>MGSSHHHHHSSGENLYFQGHMSIPFTRWPEEFARRYREKGYWQDLPLTDILTRHAASDSIAVIDGERQLSYRELNQAADNLACSLRRQGIKPGETALVQLGNVAELYITFFALLKLGVAPVLALFSHQRSELNAYASQIEPALLIADRQHALFSGDDFLNTFVTEHSSIRVVQLLNDSGEHNLQDAINHPAEDFTATPSPADEVAYFQLSGGTTGTPKLIPRTHNDYYYSVRRSVEICQFTQQTRYLCAIPAAHNYAMSSPGSLGVFLAGGTVVLAADPSATLCFPLIEKHQVNVTALVPPAVSLWLQALIEGESRAQLASLKLLQVGGAR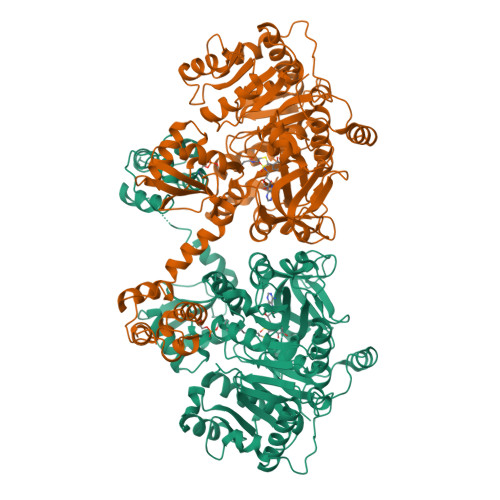LSATLAARIPAEIGCQLQQVFGMAEGLVNYTRLDDSAEKIIHTQGYPMCPDDEVWVADAEGNPLPQGEVGRLMTRGPYTFRGYYKSPQHNASAFDANGFYCSGDLISIDPEGYITVQGREKDQINRGGEKIAAEEIENLLLRHPAVIYAALVSMEDELMGEKSCAYLVVKEPLRAVQVRRFLREQGIAEFKLPDRVECVDSLPLTAVGKVDKKQLRQWLASRASAGRASIPASKAALREVILPLLDESDEPFDDDNLIDYGLDSVRMMALAARWRKVHGDIDFVMLAKNPTIDAWWKLLSREVK[2x]> MNHKVHHHHHHIEGRHMGLQVVNVEGIDFATKFAPPTSSTELDLIGHGNTGMEIETVEIRFTAMGFYAEPSISEHLQKWKGKAVSELVEDDSGFHKELIQVPVEKAVRISIIKGIKGL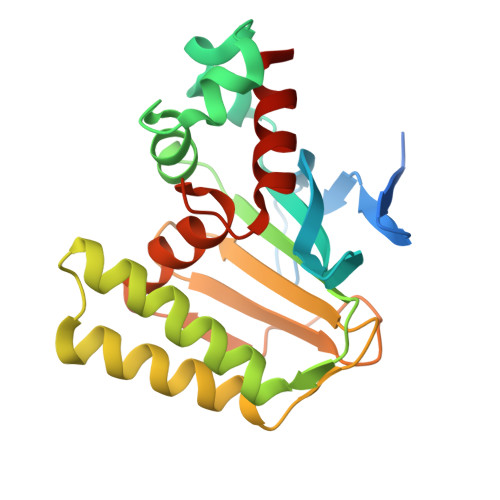PYGSALQSSLRDRLVNDDKFEEEEEEALEKLVEFFQPHNLPKGANIIYHWATPDTVKISLSEEGKIPDEVSYTIEDANVAEALLDLYLGENTITPSTLSSVAEAIAAQVA>[2x]TQNSLSTSLQRLSSGLRINSAKDDAAGLAISDRMTAQIKGLTQAQRNANDGISLAQTAEGALGEISNNLQRIRELAVQASNGTNTQTDRDALQAEVTQLQSEIQRVAEQTSFNGQKLLDGSFNGVQFQIGANAGETIGVSKIMNAQTASLGGSLTRTTSTIDATDLTKYDTAMAAGDLTINGVDVGKIDAASTAQERAAQLTEAINRVSSQ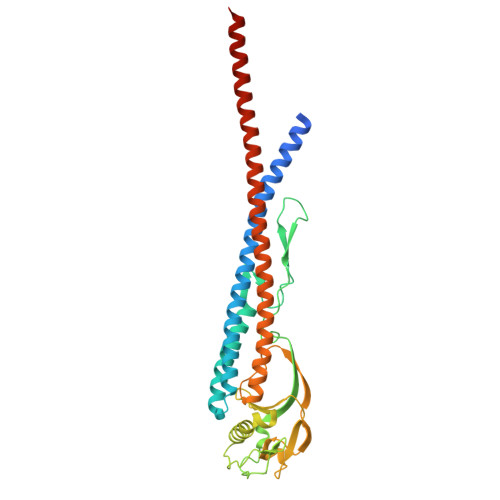TNVGASYDKTTGQVTLTSNAAIAVAGAANDATVAGWANNATTGTATTTTGINSLTVSSFTNAQQTITQIDNALKDINTARADLGAVQNRFTSTVANLQSMTENLSSARGRVTDADFASETANLSRAQILQQALEHHHHHH N-(3,3-dimethyl-3,4-dihydroisoquinolin-1-yl)-L-phenylalanine | C20 H22 N2 O2 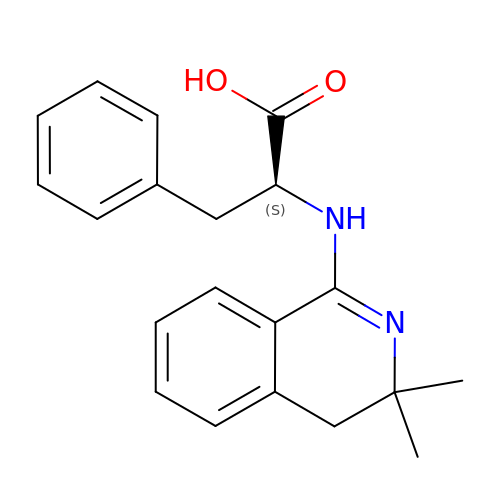| SKZOZLFDNIMQMW-KRWDZBQOSA-N7-[3-(isoquinolin-7-yloxymethyl)-1,5-dimethyl-pyrazol-4-yl]-3-(3-naphthalen-1-yloxypropyl)-1H-indole-2-carboxylic 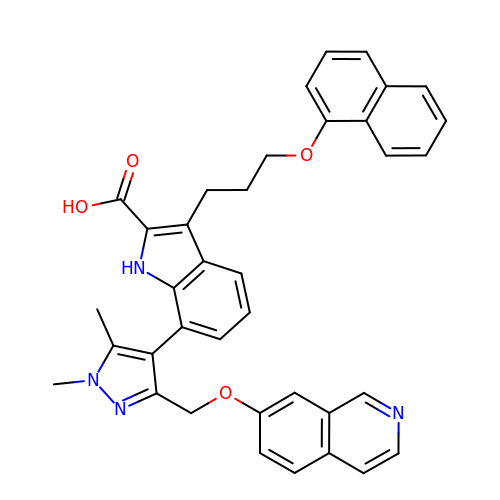acid | C37 H32 N4 O4 | AESVOHYVDHPIND-UHFFFAOYSA-N> IT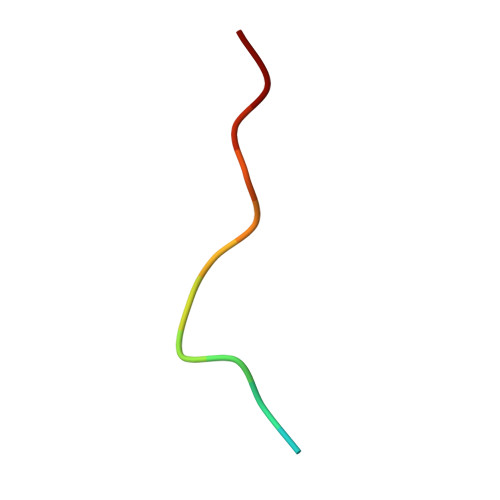GFSDDVPMVIA>[5x]GSAAAQDMVSPPPPIADEPLTVNTGIYLIESYSLDDCAETF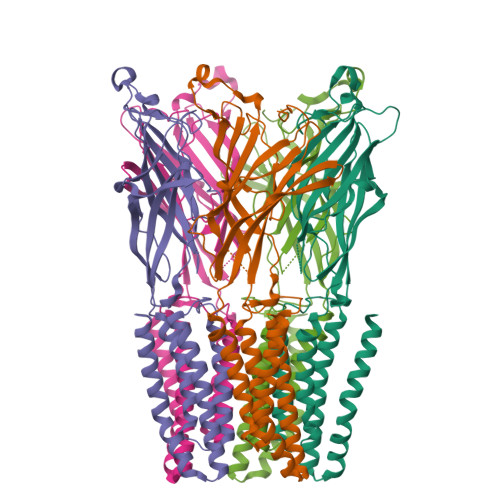KVNAFLSLSWKDRRLAFDPVRSGVRVKTYEPEAIWIPEIRFVNVENARDADVVDISVSPDGTVQYLERFSARVLSPLDFRRYPFDSQTLHIYLIVRSVDTRNIVLAVDLEKVGKNDDVFLTGWDIESFTAVVKPANFALEDRLESKLDYQLRISRQYFSYIPNIILPMLFILFISWTAFWSTSYEANVTLVVSTLIAHIAFNILVECNLPKTPYMTYTGAIIFMIYLFYFVAVIEVTVQHYLKVESQPARAASITRASRIAFPVVFLLANIILAFLFFGF>MAAESVRVAVRCRPFNQREKDLNTTLCVGMTPNVGQVNLNAPDGAAKDFTFDGAYFMDSTGEQIYNDIVFPLVENVIEGYNGTVFAYGQTGSGKTFSMQGIETIPAQRGVIPRA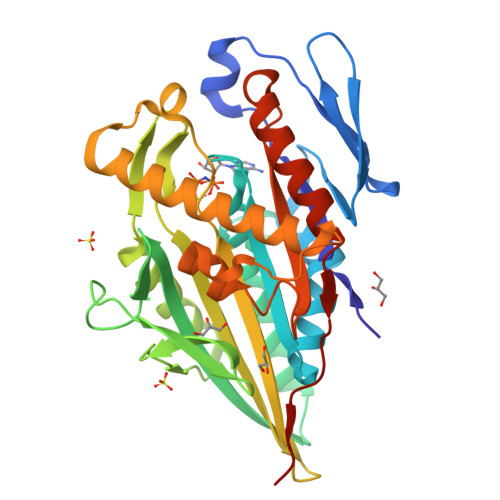FDHIFTATATTENVKFLVHCSYLEIYNEEVRDLLGADNKQKLEIKEQPDRGVYVAGLSMHVCHDVPACKELMTRGFNNRHVGATLMNKDSSRSHSIFTVYVEGMTETGSIRMGKLNLVDLAGSERQSKTGATGDRLKEATKINLSLSALGNVISALVDGKSKHIPYRDSKLTRLLQDSLGGNTKTIMIACVSPSSDNYDETLSTLRYANRAKNIKNKPTINEDPLEHHHHHH[2x]(5~{S})-5-[[2,6-bis(fluoranyl)phenyl]methoxymethyl]-3-(2-fluorophenyl)-5-methyl-4~{H}-1,2-oxazole | C18 H16 F3 N O2 | 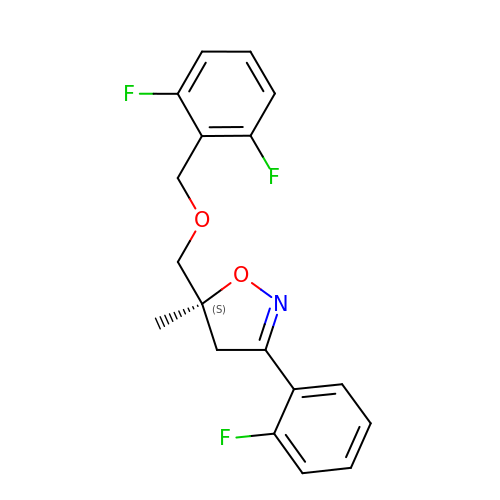ZEFIDENJKVKCIX-SFHVURJKSA-N> GPLSVAPEMDIMDYCKKEWRGNTQKATCMKMGYEEVSQKFTSIRRVRGDNYCALRATLFQAMSQAVGLPPWLQDPEL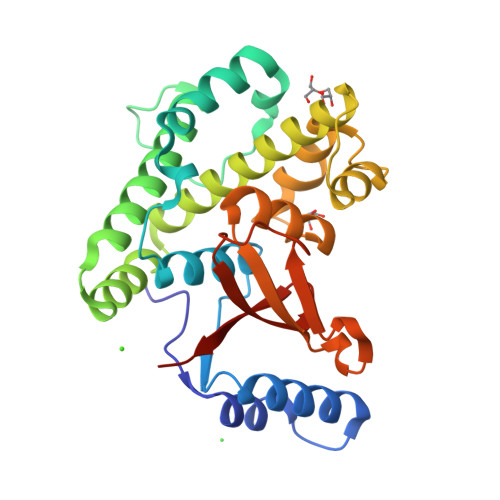MLLPEKLISKYNWIKQWKLGLKFDGKNEDLVDKIKESLTLLRKKWAGLAEMRTAEARQIACDELFTNEAEEYSLYEAVKFLMLNRAIELYNDKEKGKEVPFFSVLLFARDTSNDPGQLLRNHLNQVGHTGGLEQVEMFLLAYAVRHTIQVYRLSKYNTEEFITVYPTDPPKDWPVVTLIAEDDRHYNIPVRVCEETSL>[2x]GPGSGSEGKRLTDQLRWKIMSLKMRIEQLKQTISKLNEEMKKNSEGLL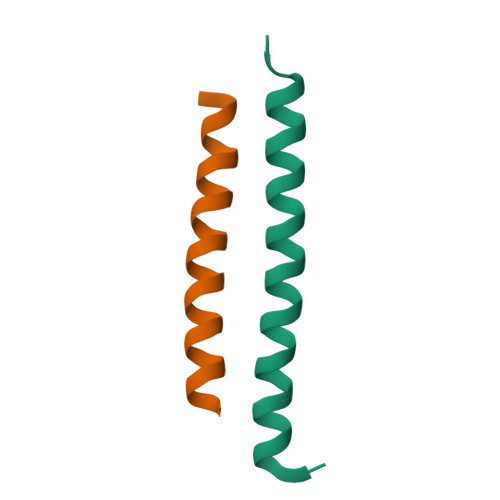KNKEKNQKLYSR;>GPGSDEAAALRAELRDLELEEARLVQELEDVDRNNARAAADLQAAQAEAAELDQQERQHYRDYSALKRQQLELLDQLGNVENQLQYARVQLDRLKE[2x]SulE, an esterase, which detoxifies a variety of sulfonylurea herbicides through de-esterification, provides an attractive approach to remove environmental sulfonylurea herbicides and develop herbicide-tolerant crops. SulE catalyzes the de-esterification of a variety of sulfonylurea herbicides, such as MM, BM, SM, TM, TrM, EM, and CE, to the corresponding herbicidal-inactive parent acid. The structures show that SulE is a dimer with a lid loop in a domain-swapped β-hairpin covering the active site from the opposing monomer. SulE shows a similar catalytic triad consisting of Ser209, His333, and Glu232 at its active site.

To understand the molecular basis for the altered activity by Pro44 mutation, the crystal structures of apo-P44R, the double mutant P44R/S209A in complex with CA, and the triple mutant P44R/S209A/H333A in complex with MM, CE, and TM were determined in the range of 1.32–1.78 Å. The lid loop conformational change could also be observed in the P44R/S209A/H333A-CE complex structure. A clear electron density was observed for full MM and CE molecule in the active site of P44R/S209A/H333A, indicating that MM and CE was tightly bound in P44R/S209A/H333A. Superimposition of S209A/H333A-CE and P44R/S209A/H333A-CE complex structures also revealed a similar conformational alteration of CE. In this position, more favorable interactions of the heterocycle moiety of MM and CE with P44R were observed. The heterocycle ring was packed against by Ile43 and Ser142 from both sides. Additionally, the conformational rotation of sulfonylurea bridge results in carbonyl oxygen atom of the bridge hydrogen-bonded with the amino group of Arg150 (about 3.0 Å), while in the original conformation, the distance between Arg150 and the oxygen atom of the sulfonyl group of MM and CE is more than 4.0 Å, beyond the canonical hydrogen bond distance. The sulfonylurea bridge also forms hydrogen bonds with several surrounding water molecules. These interactions make the heterocycle more tightly binding to the protein. In the P44R/S209A/H333A-MM and P44R/S209A/H333A-CE complex structures, because the heterocyclic ring occupies the position of the original Tyr45 side chain, we speculate that the steric hindrance of Tyr45 in wild-type SulE restricts heterocycles from entering the active pocket. The relocation of the heterocycle ring results in a more stable binding of substrate to an enzyme and further improved the activity of SulE against MM and CE.

>METDNVELAQSKRKVVLAEQGSFYIGGRTVTGPGKFDPSKPVIRYSNEGATFYINQMYVNFQAPVRPRGLPLVFWHGGGLTGHIWESTPDGRPGFQTLFVQDRHTVYTIDQPGRGRGNIPTFNGPFGQLEEESIVNTVTGNSSKEGAWVRDRLGPAPGQFFENSQFPRGYEDNYFKEMGFSPSISSDEIVDAVVKLVTHIGPCVLVTHAASGVLGMRVATHAKNVRGIVAYEPATSIFPKGKVPEIPPLADKKSQIFPPFEIQESYFKKLAKIPIQFVFGDNIPKNPKSAYWFLDWWRVTRYAHSLSLEAINKLGGQASLLDLPTAGLRGNTAFPFTDRNNVQVASLLSDFLGKHGLDQNESLEHHHHHH[2x]>[2x]RQNWEEADSMKSSVESLQNRVTELESVDKSAGQVARNTGLLESQLSRHDQMLSVHDIRLADMDLRFQVLETASYNGVLIWKIRDYKRRKQEAVMGKTLSLYSQPFYTGYFGYKMCARVYLNGDGMGKGTHLSLFFVIMRGEYDALLPWPFKQKVTLMLMDQGSSRRHLGDAFKPDPNSSSFK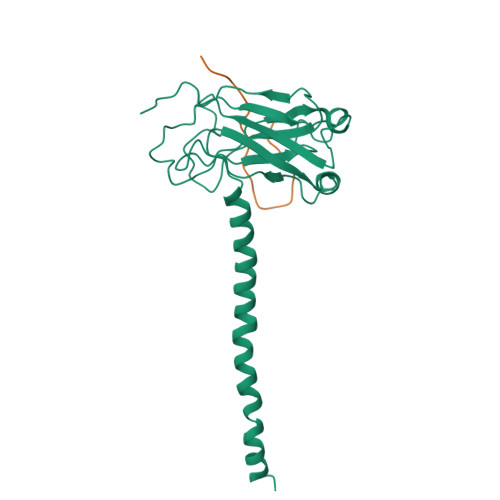KPTGEMNIASGCPVFVAQTVLENGTYIKDDTIFIKVIVDTSDLPDP;>KTAAPVQETLHGSQPVTQEDG[2x]methyl (4R)-4-amino-1-methyl-L-prolinate | C7 H14 N2 O2 | 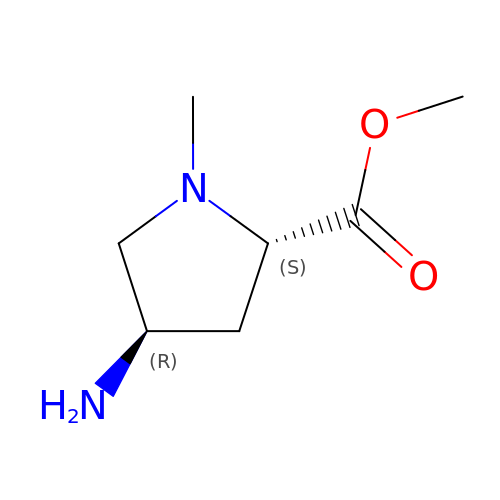WWDRZXVUQYMTLY-RITPCOANSA-N> MISEEETLVFFDLETTGLDTSRCDIVQLSAISGAQVFSVYLLPRCCITEGASQVTGLWVDGSTLMLRERPVQTVPHQQALTGFIRFLQNQTFGRPILVGHNSRRFD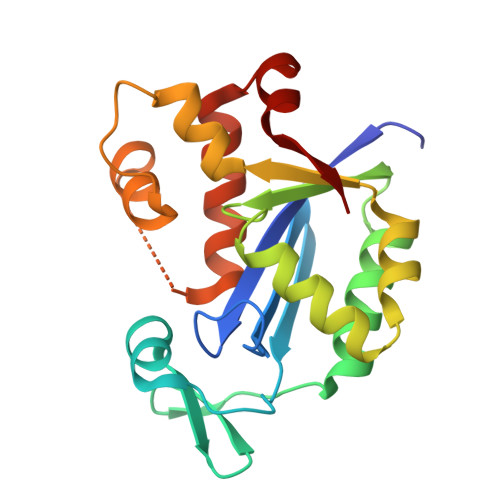WPILRRVLEEFGLLQEFRSCASECVDTLSLSREMFRNALQKFSQPFLVQHFLQQEYRAHDASEDVRTLQELYRVWRPSLELRDNHTFRL(2S,7R,9R)-4,5-dihydroxy-2,3,6,7,8,9-hexahydro-1H-pyrrolo[2,3-f]quinoline-2,7,9-tricarboxylic 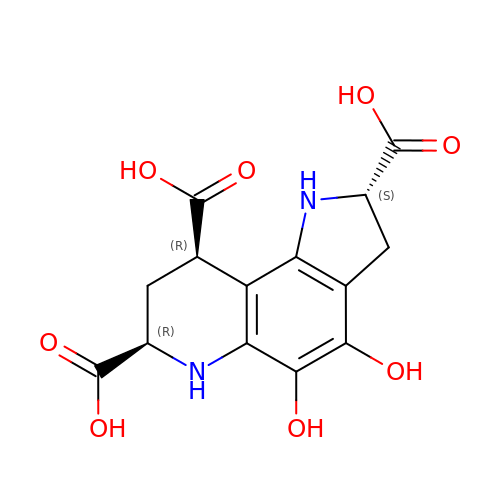acid | C14 H14 N2 O8 | AEQJGIAJKMGQCZ-PUFIMZNGSA-N>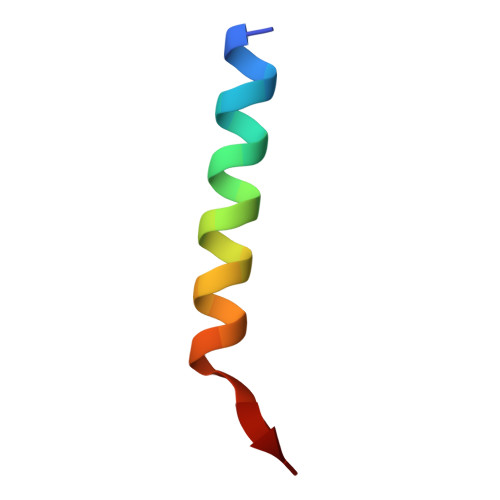 EDIIRNIARHLAQMGDSMDRSWGGC> MDYKDDDDKLAEHGESSEDRISEIDYEFLPELSALLGVDAFQVAKSQEEEEHKERMKMKKGFNSQMRSEAKRLKTFETYDTFRSWTPQEMAAAGFYHTGVRLGVQCFCCSLILFGNSLRKLPIERHKKLRPECEFLQGKDVGNIGKYDIRVKRPEKMLRGGKARYHEEEARLESFEDWPFYAHGTSPRVLSAAGFVFTGKRDTVQCFSCGGSLGNWEEGDDPWKEHAKWFPKCEFLQSKKSSEEIAQYIQSYEGFVHVTGEHFVKSWVRRELPMVSAYCNDSVFANEELRMDMFKDWPQESPVGVEALVRAGFFYTGKKDIVRCFSCGGCLEKWAEGDDPMEDHIKFFPECVFLQTLKSSAEVIPTLQSQYALPEATETTRESNHGDAAAVHSTVVDLGRSEAQWFQEARSLSEQLRDNYTKATFRHMNLPEVCSSLGTDHLLSCDVSIISKHISQPVQEALTIPEVFSNLNSVMCVEGETGSGKTTFLKRIAFLWASGCCPLLYRFQLVFYLSLSSITPDQGLANIICAQLLGAGGCISEVCLSSSIQQLQHQVLFLLDDYSGLASLPQALHTLITKNYLSRTCLLIAVHTNRVRDIRLYLGTSLEIQEFPFYNTVSVLRKFFSHDIICVEKLIIYFIDNKDLQGVYKTPLFVAAVCTDWIQNASAQDKFQDVTLFQSYMQYLSLKYKATAEPLQATVSSCGQLALTGLFSSCFEFNSDDLAEAGVDEDEKLTTLLMSKFTAQRLRPVYRFLGPLFQEFLAAVRLTELLSSDRQEDQDLGLYYLRQIDSPLKAINSFNIFLYYVSSHSSSKAAPTVVSHLLQLVDEKESLENMSENEDYMKLHPQTFLWFQFVRGLWLVSPESSSSFVSEHLLRLALIFAYESNTVAECSPFILQFLRGKTLALRVLNLQYFRDHPESLLLLRSLKVSINGNKMSSYVDYSFKTYFENLQPPAIDEEYTSAFEHISEWRRNFAQDEEIIKNYENIRPRALPDISEGYWKLSPKPCKIPKLEVQVNNTDAADQALLQVLMEVFSASQSIEFRLFNSSGFLESICPALELSKASVTKCSMSRLELSRAEQELLLTLPALQSLEVSETNQLPEQLFHNLHKFLGLKELCVRLDGKPNVLSVLPREFPNLLHMEKLSIQTSTESDLSKLVKFIQNFPNLHVFHLKCDFLSNCESLMAVLASCK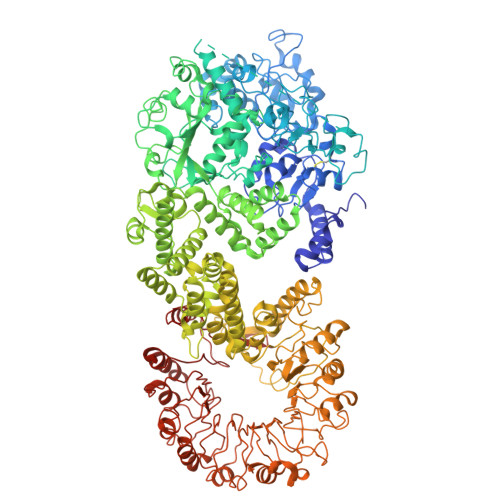KLREIEFSGRCFEAMTFVNILPNFVSLKILNLKDQQFPDKETSEKFAQALGSLRNLEELLVPTGDGIHQVAKLIVRQCLQLPCLRVLTFHDILDDDSVIEIARAATSGGFQKLENLDISMNHKITEEGYRNFFQALDNLPNLQELNICRNIPGRIQVQATTVKALGQCVSRLPSLIRLHMLSWLLDEEDMKVINDVKERHPQSKRLIIFWKLIVPFSPVILE> ECISVKGRIYSILKQIGSGGSSKVFQVLNEKKQIYAIKYVNLEEADNQTLDSYRNEIAYLNKLQQHSDKIIRLYDYEITDQYIYMVMECGNIDLNSWLKKKKSIDPWERKSYWKNMLEAVHTIHQHGIVHSDLKPANFLIVDGMLKLIDFGIANQMQPDTTSVVKDSQVGTVNYMPPEAIKDMSSSRENGKSKSKISPKSDVWSLGCILYYMTYGKTPFQQIINQIS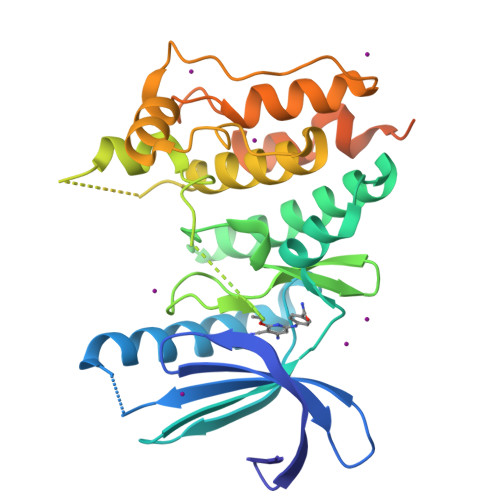KLHAIIDPNHEIEFPDIPEKDLQDVLKCCLKRDPKQRISIPELLAHPYVQIQTHPVNQMAKGTTEEMKYVLGQLVGLNLVPRGSAAGHHHHHH>FCLTLRRRYTMA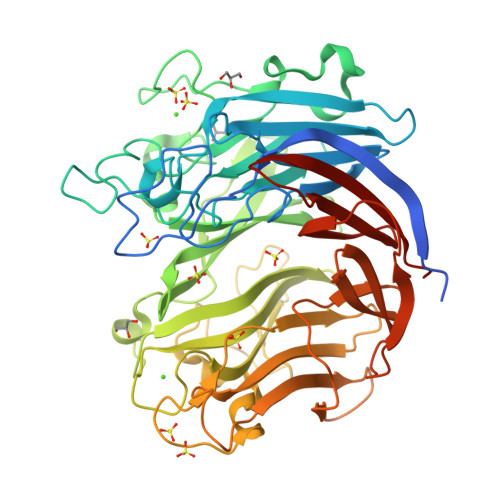NDSVSLTSNISNTSGVLLESQTKITDGALHFDGKKLNHNTFENPSKSQAYDYFFGRNISAHGDAVKPYKHFVFMTWYKGGKEERNVMLSRFNTKTGVVKTIQFPHRHTGFRGDPLVGESHNTIGLAVSPLNGTIHMVYDMHAYVDDDETGRFKGRFVDDFFRYSFSVAGAADVPDDEFTLEQFVKDTSELSQGADDYKHLTMTGNLQDKENFSALTYPKFYTSDDGELLHYMRWGGNNNGAYYFNKYDAKNQKWTRFTPFNHKDQKTHGNAYNWGLYGQMKYINGKLRVGFQQRSANNDDRFKYQNGVYYAYSDHPDGLGNWKNVDGEDMTWPLVNSDEIKIFEPGDYIDHTAPNSVHIVTGFDWTVTENDDVHFITHVRSTDTKRSDYKEVSIHAFKPANAVDFTITTDFTGADSIYTSGDSIFIIGLKNGYPFVEKAKGGSNDFEVVYQQASGVKFDHGTIHIENGKAYYYLMEKGAGNALPLHLQVIDLGVTELEHHHHHH[2x]> MKYQQLENLECGWKWAYLIRKHQEGEPITKYIENSAAHAAVDKLIKLESEPVRVLEWIEQHMNPDLFNRMKQTIRARRKRHFNAEHQHTRKKSIDLDFPVWHRLSALSQRRGNTLSETIVQLIEDAERKEK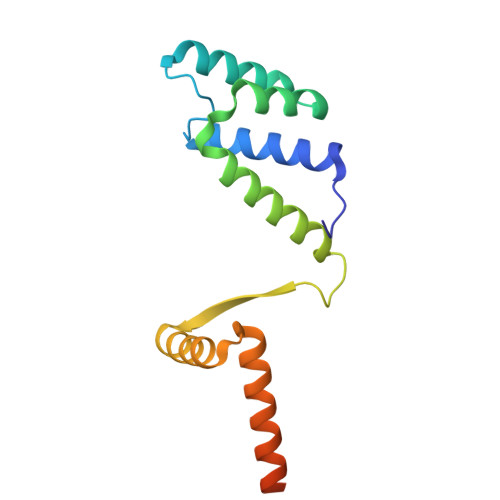YANQMSSLKHDLEAILGKNE Rad2/XPG belongs to the flap endonuclease family that encompasses various structure-specific nucleases involved in nucleic acid processing. The unique feature of Rad2/XPG is the recognition of DNA bubbles that comprise a stretch of unpaired bases flanked by double-stranded regions and correspond to the DNA in the NER pre-incision complex. We report four structures of the Rad2 catalytic core solved in four different space groups, three of which represent the productive substrate binding mode and reveal that the protein recognizes a single 5′ nucleotide of the single-stranded portion of the DNA and a 3′ phosphate group of the ss/dsDNA junction. The two critical regions for substrate binding are the H2TH module with a Rad2-specific α-helix 12b and the hydrophobic wedge that binds the first base pair of the double-stranded portion of the DNA.

Briefly, complex I comprises a Rad2-ΔSC dimer that interacts with disordered DNA. Although it may represent a functional state of the enzyme, we assume it is rather a non-productive complex. For Sc-Rad2-ΔSC in all 10 independent determinations of the structure we report herein (including the non-catalytic dimer), helix α5 is missing. However, α4 has a similar location in all 10 protein structure determinations from four different space groups, implying that the conformation we observed is stable.

>[2x]SMGVHSFWDIAGPTARPVRLESLEDKRMAVDASIWIYQFLKAVRDQEGNAVKNSHITGFFRRICKLLYFGIRPVFVFDGGVPVLKRETIRQRKERRQGKRESAKSTARKLLANTTLSTSAERNVAENAFVEDELFEQQMKDKRDSDEVTMDMIKEVQELLSRFGIPYITAPMEAEAQCAELLQLNLVDGIITDDSDVFLFGGTKIYKNMFHEKNYVEFYDAESILKLLGLDRKNMIELAQLLGSDYTNGLKGMGPVSSIEVIAEFGNLKNFKDWYNNGQFDKRKQETENKFEKDLRKKLVNNEIILDDDFPSVMVYDAYMRPEVDHDTTPFVWGVPDLDMLRSFMKTQLGWPHEKSDEILIPLIRDV> MEELDVDPAETPIPGLGQQNRHIGFSWGPGDLLLYETLYQKQGNSETAARCPFMYLVRSDEDIYSPVLRKLFNESHSIFVGLQKSAEEASGKSRKAQLVQVSRNYRSVLRACMEEMHTLSESTRETAQKYISQISILSAMELSWNLCEILFIESAPAGPLLILLLEWVRLHVCEVDNIVQDVLRSEKPTEHEKFWDGVTGYVLQGRMNEARQLLAKEASTSASARSMCRVLDDLLKKMPMLHTGGTQTLTEFELKWQHWREECERHLQNGTFSSNVHMEAVCRVLLGDEEVLLEKRDLMTTWYHFLVSRLLFKHPTVKPTELHFYAQSSLDMFLAGDSCPEPLDNILLAAFEFDI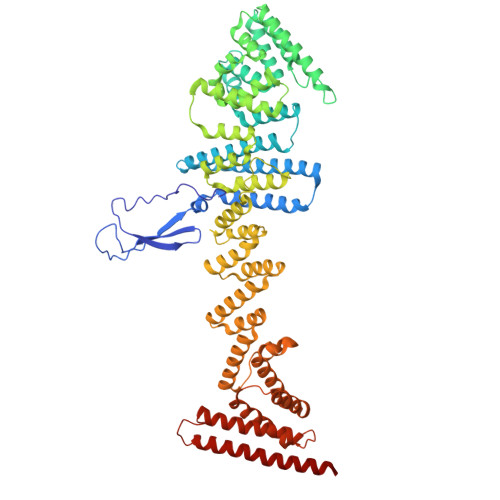HQVIKEFSIVSSNWWFVAHLTDLLDHCQLFQAHNLYFGANMREFLLLDYASGLFSHHSLWQLGVDYFDYCPNLGREYLKLHMERIPLSTEKKALKALRICEQRQMTEQVRSICKTMAMQSLCNRRLGSALSWSIRAKDAAFATLISDRFLKEYCERGNFTDLDLIDNLGSAMLLSDRLTFLGKYREFHRMYSQEQFSEAASLLLSLMTARIAPCSFWLTLLLDALPLLEQKQVIFSAEQTYELMRCLEDRMAAKLESTSPDEIQKQDSSIDNTKVEMLRLALARNLARAIVTEGALQE> MFLLQAPL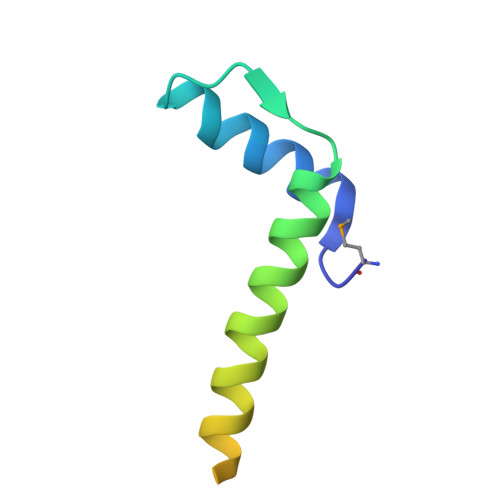QRRILEIGKKHGITELHPDVVSYVSHATQQRLQNLVEKISETAQQKNFSYKDDDRYEQASDVRAQLK>GSDEDTYYLQVRGRENFEILMKLKESLELMELVP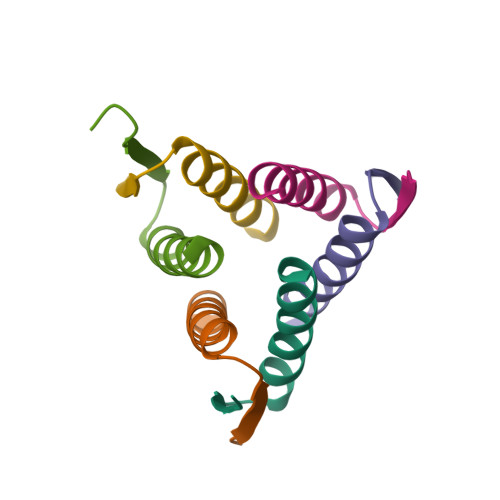Q[28x]> RIPGFDISGWQPTTDFARAYANGDRFVYIKATEGTTFKSSAFSRQYTGATQNGFIRGAYHFAQPAASSGAAQARYFASNGGGWSKDGITLPGALDIEYNPNGATCYGLSQSAMVNWIEDFVTTYHGITSRWPVIYTTTDWWTQCTGNSNRFANRCPLWIARYASSVGTLPNGWGFYTFWQYNDKYPQG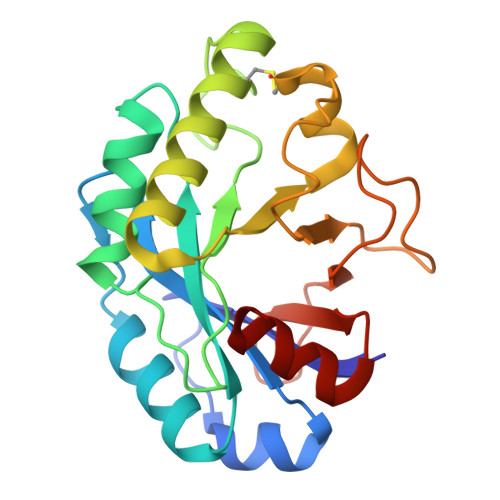GDSNWFNGDASRLRALANGD>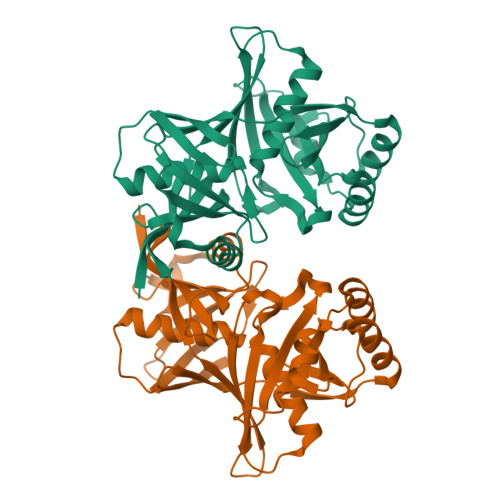 MTLMVPFKQVDVFTEKPFMGNPVAVINFLEIDENEVSQEELQAIANWTNLSETTFLFKPSDKKYDYKLRIFTPRSELPFAGHPTIGSCKAFLEFTKNTTATSLVQECKIGAVPITINEGLISFKAPMADYESISSEMIADYEKAIGLKFIKPPALLHTGPEWIVALVEDAETCFNANPNFAMLAHQTKQNDHVGIILAGPKKEAAIKNSYEMRAFAPVINVYEDPVCGSGSVALARYLQEVYKFEKTTDITISEGGRLKRNGLMLASIKKEADNSTSYYIAGHATTVIDGKIKVHHHHHH> MGSDKIHHHHHHMKIDILDKGFVELVDVMGNDLSAVRAARVSFDMGLKDEERDRHLIEYLMKHGHETPFEHIVFTFHVKAPIFVARQWFRHRIASYNELSGRYSKLSYEFYIPSPERLEGYKTTIPPERVTEKISEIVDKAYRTYLELIESGVPREVARIVLPLNLYTRFFWTVNARSLMNFLNLRADSHAQWEIQQYALAIA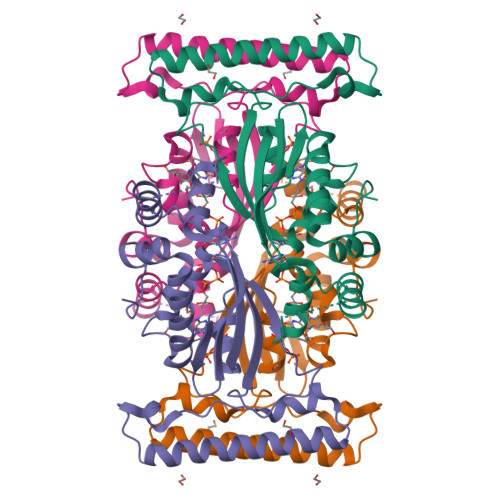RIFKEKCPWTFEAFLKYAYKGDILKEVQV>YKKAGLQRTLVLIKPDAFERSLVAEIMGRIEKKNFKIVSMKFWSKAPRNLIEQHYKEHSEQSYFNDLCDFMVSGPIISIVYEGTDAISKIRRLQGNTNPLASAPGTIRGDLANDIGENLIHASDSEDSAVDEISIWF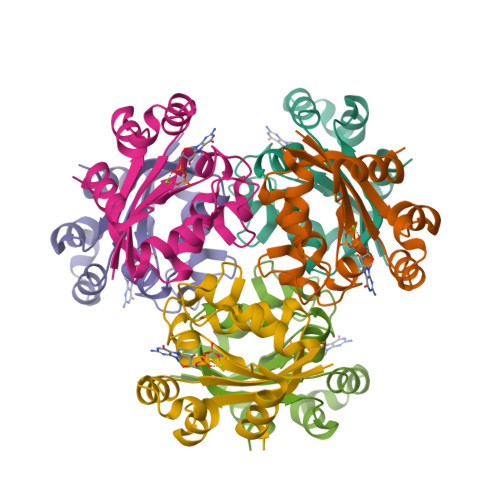PETKMETDN[2x]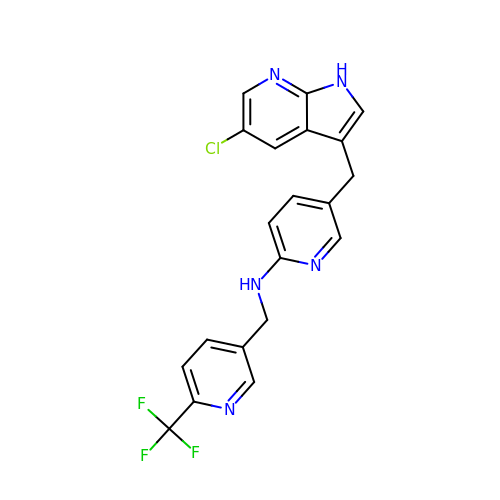5-[(5-chloro-1H-pyrrolo[2,3-b]pyridin-3-yl)methyl]-N-{[6-(trifluoromethyl)pyridin-3-yl]methyl}pyridin-2-amine | C20 H15 Cl F3 N5 | JGWRKYUXBBNENE-UHFFFAOYSA-N>[2x]GHMENKVINFKKIIDSRGSLVAIEENKNIPFSIKRVYYIFDTKGEEPRGF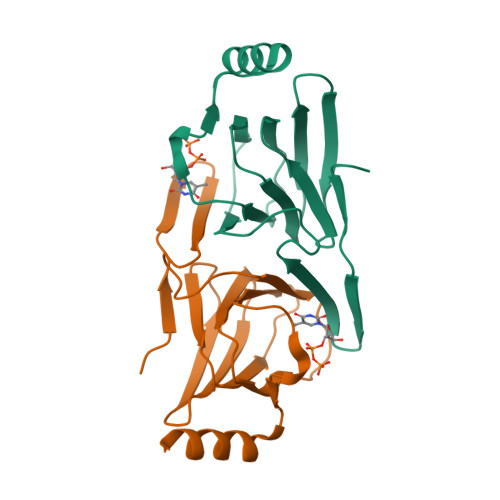NANKKLEQVLVCLNGSCRVILDDGNIIQEITLDSPAVGLYVGPAVWHEMHDFSSDCVMMVLASDYYDETDYIRQYDNFKKYIAKINLEKEG> HPETLVKVKDAEDQLGARVGYIELDLNSGKILESFRPEERFPMMSTFKVLLCGAVLSRVDAGQEQLGRRIHYSQNDLVEYSPVTEKHLTDGMTVRELCSAAITMSDNTAANLLLTTIGGPKELTAFLHNMGDHVTRLDRWEPELNEAIPNDERDTTMPAAMATTLRKLLTGELLTLASRQQLIDWMEADKVAGPLLRSALPAGWFIADKSGAGERGSRGIIAALGPDGKPSRIVVIYTTGSQATMDERNRQIAEIGASLI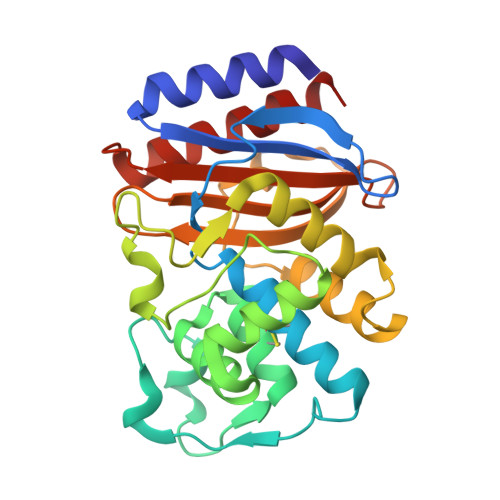KHW> MAILDLKSLVMNAINYWGPKNNNGIQGGDFGYPISEKQIDTSIITFTHPRLIPYDLTIPQNLETIFTTTQVLTNNTDLQQSQTVSFAKKTTTTTSTSTTNGWTEGGKISDTLEEKVSVSIPFIGEGGGKNS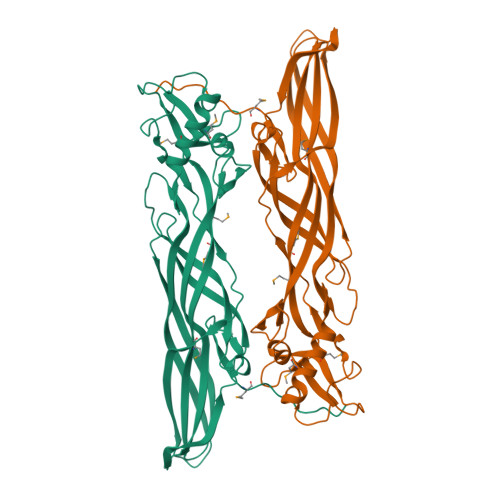TTIEANFAHNSSTTTFQQASTDIEWNISQPVLVPPSKQVVATLVIMGGNFTIPMDLMTTIDSTEHYSHYSGYPILTWISSPDNSYSGPFMSWYFANWPNLPSGFGPLNSDNTVTYTGSVVSQVSAGVYATVRFDQYDIHNLRTIEKTWYARHATLHNGKKISINNVTEMAPTSPIKTN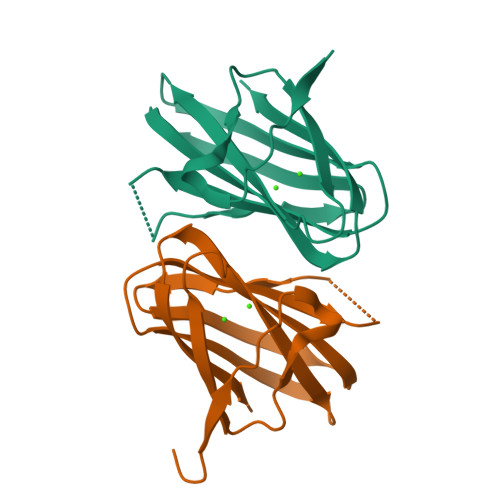>[2x]GSPGIPGNEKLKEKENNDSSDKATVIPNFNTTMQGSLLGDDSRDYYSFEVKEEGEVNIELDKKDEFGVTWTLHPESNINDRITYGQVDGNKVSNKVKLRPGKYYLLVYKYSGSGNYELRVNK>GSSLQRYEKLVKECRRLEEELEQKTHEASDASQRVRQLERETTRLMRRVEQLVSAVEGQKQKLDETEAKHKLELAEIENRHELEIQSKMSSHEEALRRLMDARR[2x]

Kinetoplastids (such as Trypanosoma brucei), a group of evolutionarily divergent eukaryotes, have a unique set of kinetochore proteins that lack any significant homology to canonical kinetochore components. We previously identified KKT4 as a microtubule-binding kinetochore protein in T. brucei (throughout this manuscript we refer to KKT4 from Trypanosoma brucei unless stated otherwise) (Llauro et al., 2018). KKT4 directly binds to microtubules and maintains load-bearing attachments to both growing and shortening microtubule tips in vitro. KKT4 has the following predicted regions conserved among kinetoplastid species: an N-terminal α helix, a coiled-coil region and a block of basic residues in the microtubule-binding domain, and a BRCT domain at the C terminus.

Although we still failed to obtain diffraction-quality crystals from T. brucei, a crystal structure of KKT4117–218 from T. cruzi was solved at 1.9 Å resolution. TcKKT4117–218 is homologous to KKT4120–224 in T. brucei. The structure consists of two ∼150 Å long parallel α helices organized in a left-handed coiled-coil dimer; the helical structure starts at L118 and ends at D215. The coiled coil consists of eight regular heptad repeats starting at Y121 and ending at K176. Analysis with TWISTER shows that the six central heptads are characterized by an inter-helical distance of 4.84 ± 0.06 Å and a coiled-coil pitch (the periodicity of the coiled coil) of 136 ± 26 Å; this pitch is close to the theoretical value of 135 Å for a coiled coil. If the first and eighth heptad are included, the pitch increases to 163 ± 60 Å, indicating less supercoiling in these terminal heptads. Superposition of the coiled coils from T. cruzi and L. mexicana revealed a good structural match with a root-mean-square deviation (RMSD) of 1.03 Å (for 123 Cα), confirming the conservation of the coiled-coil structure in these species. Instead, we observed elevated B factors for the region where we might expect to find an unstructured linker in the TcKKT4 structure based on the sequence alignment. Unlike T. brucei KKT4, the coiled-coil fragments from T. cruzi and L. mexicana that were used in our structural analysis (TcKKT4117–218 and LmKKT4184–284) failed to bind microtubules in our co-sedimentation assay. A homology model for the two coiled-coil regions of T. brucei KKT4115–232 was built using the T. cruzi coiled-coil X-ray structure, and the sequence alignments confirmed using the RDC data.> ATFEIVNRCSYTVWAAASKGDAALDAGGRQLNSGESWTINVEPGTNGGKIWARTDCYFDDSGSGICKTGDCGGLLRCKRFGRPPTTLAEFSLNQYGKDYIDISNIKGFNVPMDFSPTTRGCRGVRCAADIVGQCPAKLKAPGGGCNDACTVFQTSEYCCTTGKCGPTEYSRFFKRLCPDAFSYVLDKPTTVTCPGSSNYRVTFC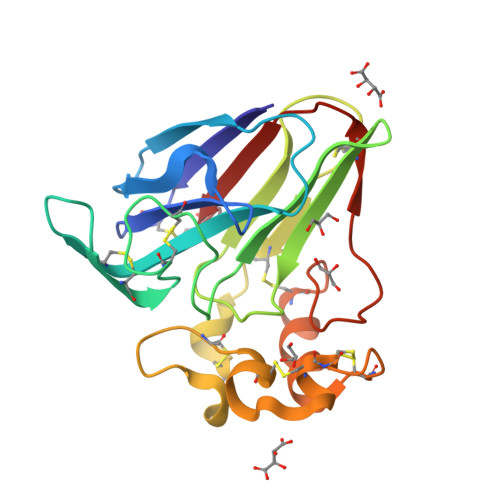PT>VLPENMKRYMGRDAQRMNILAGRIIAETVRSTLGPKGMDKMLVDDLGDVVVTNDGVTILREMSVEHPAAKMLIEVAKTQEKEVGDGTTTAVVVAGELLRKAEELLDQNVHPTIVVKGYQAAAQKAQELLKTIACEVGAQDKEILTKIAMTSITGKGAEKAKEKLAEIIVEAVSAVVDDEGKVDKDLIKIEKKSGASIDDTELIKGVLVDKERVSAQMPKKVTDAKIALLNCAIEETASEMLKDMVAEIKASGANVLFCQKGIDDLAQHYLAKEGIVAARRVKKS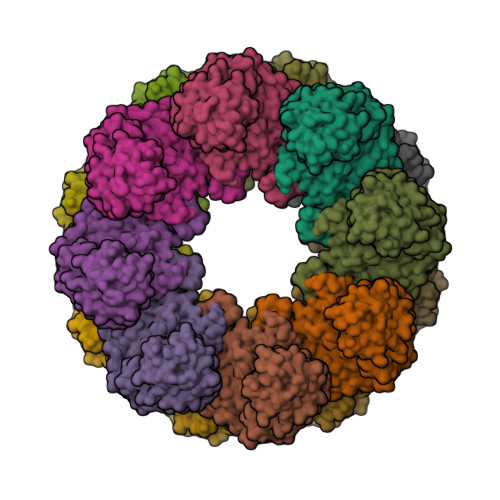DMEKLAKATGANVITNIKDLSAQDLGDAGLVEERKISGDSMIFVEECKHPKAVTMLIRGTTEHVIEEVARAVDAAVGVVGCTIEDGRIVSGGGSTEVELSMKLREYAEGISGREQLAVRAFADALEVIPRTLAENAGLDAIEILVKVRAAHASNGNKCAGLNVFTGAVEDMCENGVVEPLRVKTQAIQSAAESTEMLLRIDDVIAAE[16x]>GSSGSSGVQFDVTIEIPKGQRNKYEVDHETGRVRLDRYLYTPMAYPTDYGFIEDTLGDDGDPLDALVLLPQPVFPGVLVAARPVGMFRMVDEHGGDDKVLCVPAGDPRWDHVQDIGDVPAFELDAIKHFFVHYKDLEPG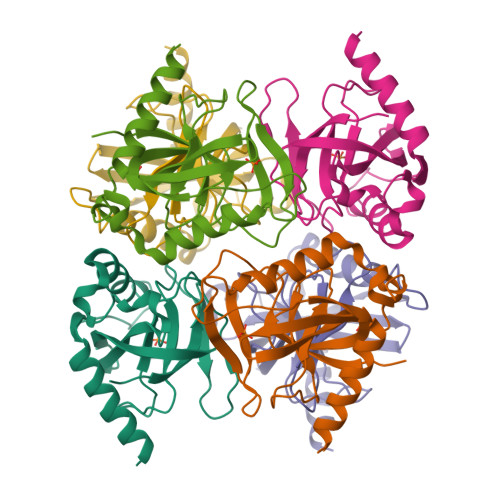KFVKAADWVDRAEAEAEVQRSVERFKAGTH[3x]> MKHHHHHHMKQNSPLDEENLTQENQDRGTHVDRGLASANVDFAFSLYKQLVLKAPDKNVIFSPLSISTALAFLSLGAHNTTLTEILKGLKFNLTETSEAEIHQSFQHLLRTLNQSSDELQLSMGNAMFVKEQLSLLDRFTEDAKRLYGSEAFATDFQDSAAAKKLINDYVKNGTRGKITDLIKDLDSQTMMVLVNYIFFKAKWEMPFDPQDTHQSRFYLSKKKWVMVPMMSLHHLTIPYFRDEELSCTVVQLNYTGNASALFILPDQDKMEEVEAMLSRETLARWGDSLEFREIGELYLPKFSISRDYNLNDILLQLGIEEAFTSKADLSGITGARNLAVSQV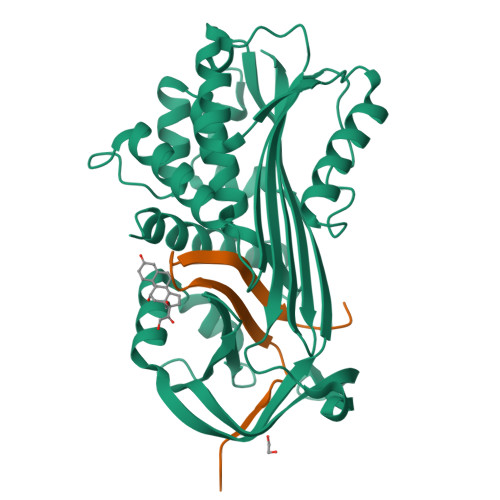VHKAVLDVFEEGTEASAATAVKITLL;> SALVETRTIVRFNRPFLMIIVDHFTWSIFFMSKVTNPKQA> GNFEEVPRETAIQFKPPLYRQRYQFVKNLVDQHEPKKVADLGCGDTSLLRLLKVNPCIELLVGVDINEDKLRWRGDSLAPFLGDFLKPRDLNLTITLYHGSVVERDSRLLGFDLITCIELIEHLDSGDLARFPEVVFGYL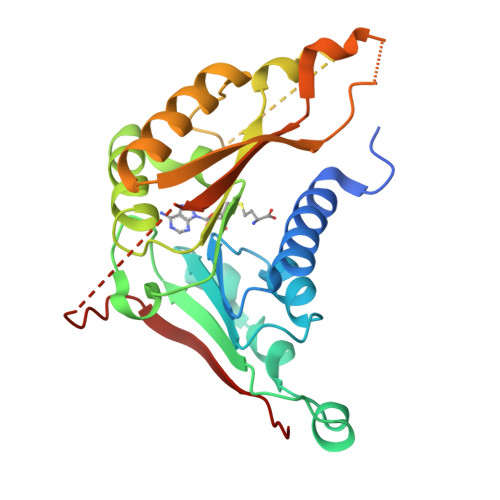SPSMIVISTPNSEFNPLFPSVTLRDSDHKFEWTRMEFQTWALYVANRYDYSVEFTGVGEPPAGAENVGYCTQIGIFRKNGGKATESCLSEQHDQHVYKAVFTTSYPSLQ>GPLGSAFENASTSVAASQMRNALNALAETVPDPEEKKRFEAEMDNFFALFRRFLNDKAKGNVVNWDRINPPAPNQVVDYNDLGAEASVEFLNKLAVVKLNGGLGTSMGCVGPKSVIEVREGMSFLDLSVRQIEHLNRTYNVNVPFVLMNSFNTDQDTQSIIKKYQGHNVDIITFNQSRYPRIIKDSLLPAPKSFDAPLQDWYPPGHGDVFESLYNSGTLDKLLERGVEYIFLSNADNLGAVVDLRILQHMADTGAEYIMELTDKTKADVKGGTIIDYEGKARLLEIAQVPKEHVNEFKSIKKFKYFNTNNIWMSLRAIKRVVEENELEMEIIANEKSIPADKKGEADQAIYQLETAVGAAIRHFKNAHGVNVPRRRFLPVKTCSDLLLVKSDLYRLEHGQLVMDPNRFGGVPVIKLGSDFKKVSDFQKRIPSIPRIVELDHLTITGAVNLGRNV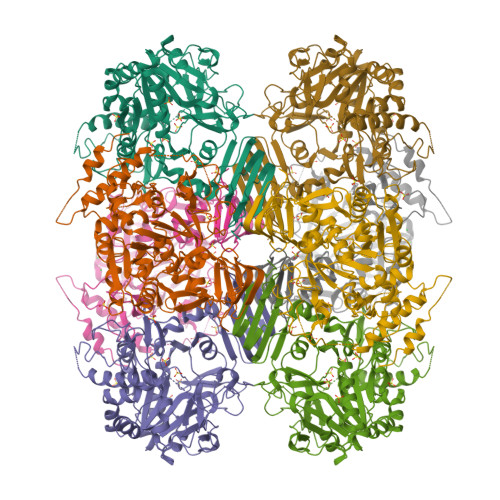TLKGTVIIVATEGSTIDIPPGSVLENCVVQGSLRILEH[2x]>[4x]MGSDKIHHHHHHENLYFQGMTFSKELREASRPIIDDIYNDGFIQDLLAG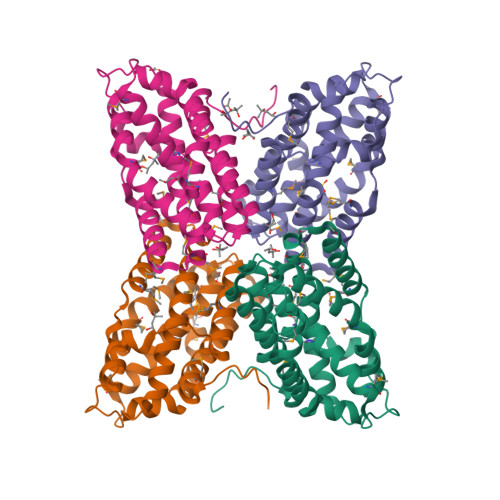KLSNQAVRQYLRADASYLKEFTNIYAMLIPKMSSMEDVKFLVEQIEFMLEGEVEAHEVLADFINEPYEEIVKEKVWPPSGDHYIKHMYFNAFARENAAFTIAAMAPCPYVYAVIGKRAMEDPKLNKESVTSKWFQFYSTEMDELVDVFDQLMDRLTKHCSETEKKEIKENFLQSTIHERHFFNMAYINEKWEYGGNNNE O-((((N-PHENYL-METHOXY-CARBONYL)-PHENYL ALANYL-CARBONYL)AMINO)-ISOBUTYL)HYDROXY PHOSPHINYL)-3-PHENYLACETIC ACID | C30 H35 N2 O8 P | 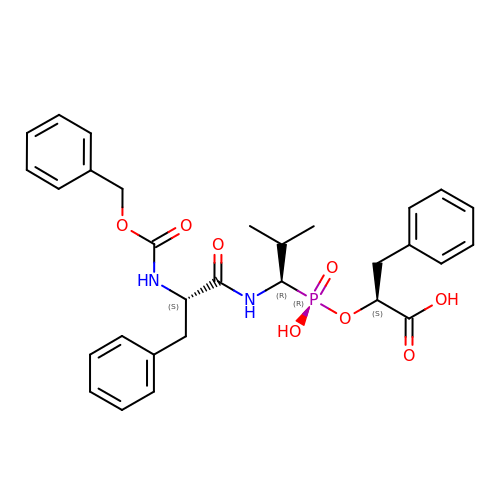NXIYKBRAJXXOLO-UNCTUWKVSA-N> SLTRIDHIGIACHDLDATVEFYRATYGFEVFHTEVNEEQGVRQAMLKINDTSDGGASYLQLLEPTREDSAVGKWLAKNGEGVHHIAFGTADVDADAADIRDKGVRVLYDEPRR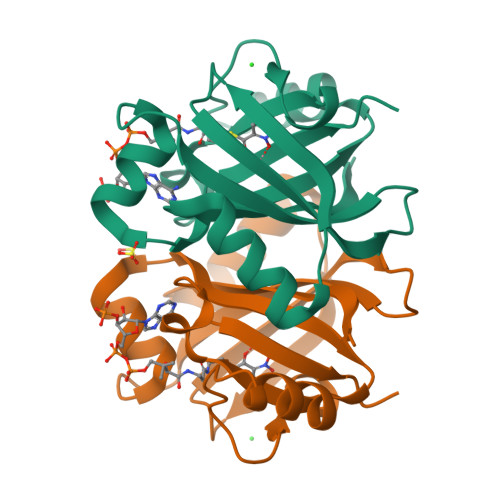GSMGSRITFLHPKDCHGVLTELVTSAAVESPEH> GPHMPEKLEAILIPDQGYHQVGPADLCTDMFVLSVTVAFATKLEQLVPSTMKLSAEGSEFFFYYSLLGNDITSEPFHNLLSPDFEPERASVRIRSSKQILKAFLSQQPSLQIHLCCGNHSLGSTDVSLSALAGISTDLDNKAATVESAFILQPPKRVKQTLPALPTDLQPTLGVAVTLRREEVALQQSVGNK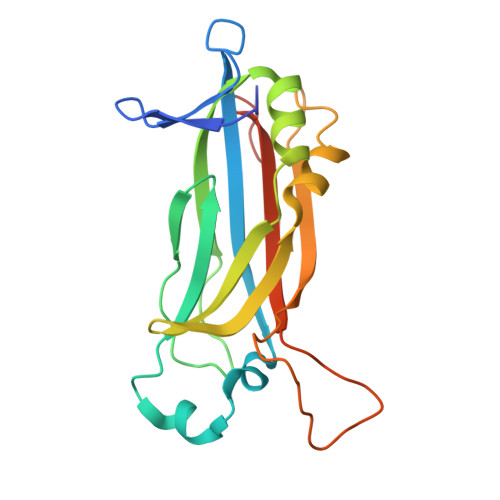E>DEPRILEAPAPDARRVYVNDPAHFAAVTQQFVIDGEAGRVIGMIDGGFLPNPVVADDGSFIAHASTVFSRIARGERTDYVEVFDPVTLLPTADIELPDAPRFLVGTYPWMTSLTPDGKTLLFYQFSPAPAVGVVDLEGKAFKRMLDVPDCYHIFPTAPDTFFMHCRDGSLAKVAFGTEGTPEITHTEVFHPEDEFLINHPAYSQKAGRLVWPTYTGKIHQIDLSSGDAKFLPAVEALTEAERADGWRPGGWQQVAYHRALDRIYLLVDQRDEWRHKTASRFVVVLDAKTGERLAKFEMGHEI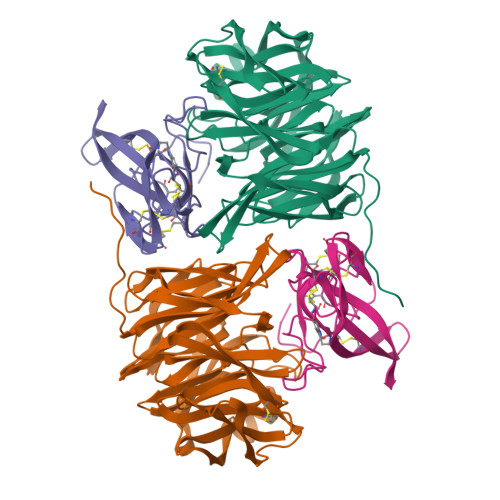DSINVSQDEKPLLYALSTGDKTLYIHDAESGEELRSVNQLGHGPQVITTADMG[2x];>[2x]TDPRAKWVPQDNDIQACDYWRHCSIDGNICDCSGGSLTNCPPGTKLATASWVASCYNPTDGQSYLIAYRDCCGYNVSGRCPCLNTEGELPVYRPEFANDIIWCFGAEDDAMTYHCTISPIVGKAS CYCLOPENTANE-1,3-DIONE 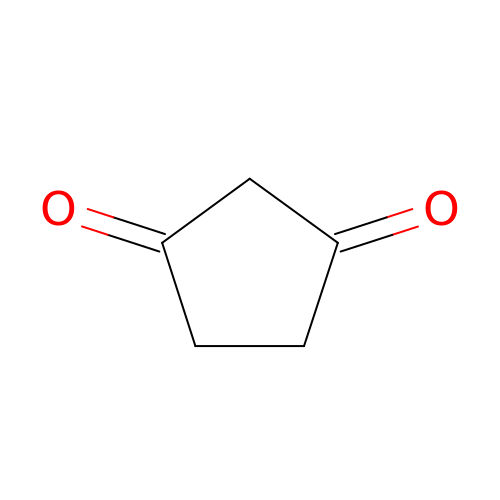| C5 H6 O2 | LOGSONSNCYTHPS-UHFFFAOYSA-N> MTELKLIHIFTDGSCLGNPGPG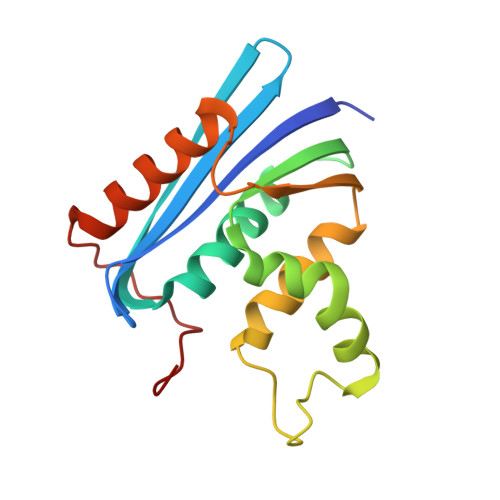GYGIVMNYKGHTKEMSDGFSLTTNNRMELLAPIVALEALKEPCKIILTSDSQYMRQGIMTWIHGWKKKGWMTSNRTPVKNVDLWKRLDKAAQLHQIDWRWVKGHAGHAENERCDQLARAAAEANPTQIDTGYQAES> SWQTYVDTNLVGTGAVTQAAILGLDGNTWATSAGFAVTPAQGTTLAGAFNNADAIRAGGFDLAGVHYVTLRADDRSIYGKKG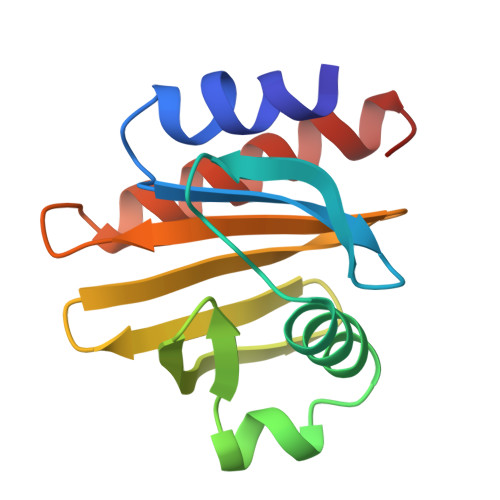SSGVITVKTSKAILVGVYNEKIQPGTAANVVEKLADYLIGQGF The small unsaturated hydrocarbon is detected by a family of receptors (ETRs) located in the membrane of the endoplasmic reticulum, which rely on a monovalent copper cofactor to detect this hydrocarbon. The copper-transporting P-type ATPase RAN1 (HMA7), located in the same membrane, is known to be essential for the biogenesis of ETRs. The AlphaFold2 model also predicts three domains at the N-terminal end, all with ATX1-like folds (henceforth referred to as MBDs) and a Cα atom RMSD < 1 Å with respect to each other. MBD3 may function as an anchor, stabilizing the RAN1-ETR1 complex while MBD1 and MBD2 are involved in a copper relay system.

To corroborate the AlphaFold2 23,28 prediction of a third ATX1-like fold domain at the N-terminus of RAN1, we expressed, purified, and analyzed this predicted domain by X-ray crystallography. The obtained crystal of the RAN1 MBD3 from Arabidopsis thaliana belongs to the orthorhombic space group P21221 with unit cell constants a = 50.755 Å, b = 51.481 Å, c = 62.722 Å. The crystal structure was determined by molecular replacement (MR) using the AlphaFold2 23,28 prediction of RAN1 (AlphaFold DB: Q9S7J8) cut to the sequence of MBD3 as a template. The structure was refined to a resolution of 1.98 Å with Rfree = 23.5% and Rwork = 19.2%, and MBD3 of RAN1 was modeled to completeness. The asymmetric unit comprises two molecules with an overall structural similarity (mutual RMSD = 0.355 Å; RMSDs to the AlphaFold2 model = 0.501/0.641 Å). The obtained crystal structure of MBD3 is consistent with the structure predicted by AlphaFold2 (Cα atom RMSD < 1 Å). However, the third domain (MBD3), which is the most distant from the N-terminus and the closest to the transmembrane domain, lacks the typical CBM. The cysteines have been substituted with asparagine and aspartate, in accordance with the results of sequence analysis by a multiple sequence alignment using Clustal Omega33. Noteworthy, a structurally related SxxS (SSRS) sequence motif is present in a loop region and α-helix 2 close to the C-terminus on the opposite side of the protein. Notably, MBD3 also showed copper-binding, with an EC50 MBD3 = 9.7 ± 1.1 µM.

>MGHHHHHHHHHHSSGHENLYFQGQQDKLVLRVDGILNELDAQVLEGILTRLNGVRQFRLDRISGELEVVFDPEVVSSRSLVDGIEEDGFGKFKLRVMSPY[2x]> GDRVADVIESSIGDSVSRALTQALPAPTGQNTQVSSHRLDTG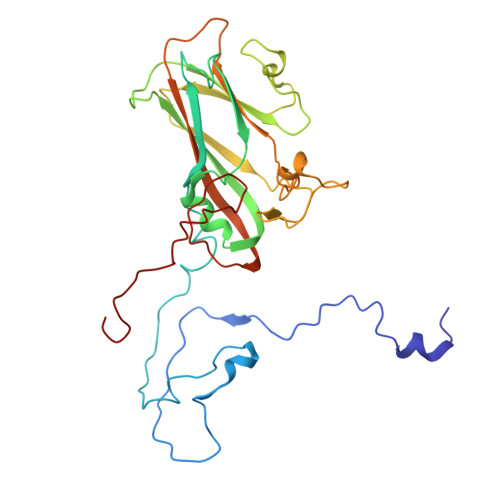EVPALQAAEIGASSNTSDESMIETRCVLNSHSTAETTLDSFFSRAGLVGEIDLPLEGTTNPNGYANWDIDITGYAQMRRKVELFTYMRFDAEFTFVACTPTGQVVPQLLQYMFVPPGAPKPESRESLAWQTATNPSVFVKLTDPPAQVSVPFMSPASAYQWFYDGYPTFGEHKQEKDLEYGACPNNMMGTFSVRTVGSSKSKYPLVVRIYMRMKHVRAWIPRPMRNQNYLFKANPNYAGNSIKPTGTSRSAITTL>XYSPTS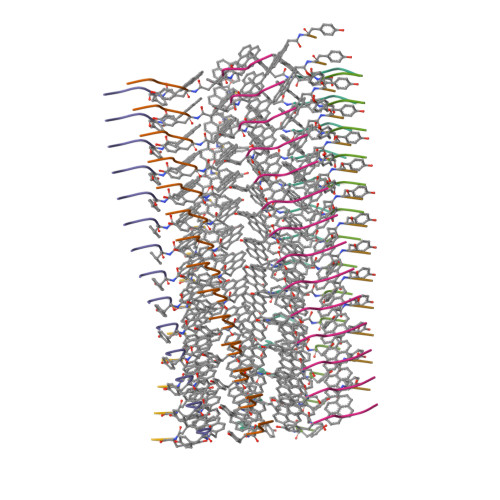PS[7x]>[2x]MSNSYEGCGDLTIFVAVALNKVIGHKNQIPWPHITHDFRFLRNGTTYIPPEVLSKNPDIQNVVIFGRKTYESIPKASLPLKNRINVILSRTVKEVPGCLVYEDLSTAIRDLRANVPHNKIFILGGSFLYKEVLDNGLCDKIYLTRLNKEYPGDTYFPDIPDTFEITAISPTFSTDFVSYDFVIYERKDCKTVFPDPPFDQLLMTGTDISVPKPKYVACPGVRIRNHEEFQYLDILADVLSHGVLKPNRTGTDAYSKFGYQMRFDLSRSFPLLTTKKVALRSIIEELLWFIKGSTNGNDLLAKNVRIWELNGRRDFLDKNGFTDREEHDLGPIYGFQWRHFGAEYLDMHADYTGKGIDQLAEIINRIKTNPNDRRLIVCSWNVSDLKKMALPPCHCFFQFYVSDNKLSCMMHQRSCDLGLGVPFNIASYSILTAMVAQVCGLGLGEFVHNLADAHIYVDHVDAVTTQIARIPHPFPRLRLNPDIRNIEDFTIDDIVVEDYVSHPPIPMAMSA

In this work, we describe the structural features of dihydrofolate reductase-thymidylate synthase from B. bovis (BbDHFR-TS), the causative agent of babesiosis in cattle. BbDHFR-TS is a homodimer that exhibits the classical dimeric interface seen in other structures of ThyA thymidylate synthase and bifunctional DHFR-TS enzymes. This 511-residue, 58.2 kDa bifunctional enzyme consists of a di­hydrofolate reductase (DHFR) subunit at the N-terminus and a thymidylate synthase (TS) subunit at the C-terminus connected by a linker. BbDHFR-TS is an obligate dimer, with two arginine side chains (Arg373′ and Arg374′) from a flexible loop in one protomer making contact with the terminal phosphate of the substrate dUMP in the opposite protomer.

Pemetrexed and raltitrexed are folate analogs designed as antitumour agents and currently approved for use in some countries for treatment of cancer. Depending on the source organism, raltitrexed has a twofold to 50-fold higher activity against TS versus DHFR, while pemetrexed tends to inhibit both enzymes equally well. The two complex structures of BbDHFR-TS have two ligands bound to each subunit of each protomer in the asymmetric unit. When both protomers from each BbDHFR-TS homodimer are compared, the complexed states reveal very similar modes of binding for both drugs to the TS subunit. The pteroyl-like groups of pemetrexed and raltitrexed are parallel to the uracil ring of dUMP when bound, mimicking the pteridine ring of the native cofactor mTHF. Although the ϕ angle of the C-terminal Ala511 in one protomer of the raltitrexed complex is rotated by approximately 30° relative to the other, this has no effect on the virtually identical binding modes of raltitrexed in both TS subunits in a single crystal structure. Both drug molecules are also observed in the DHFR subunit but appear to bind this substrate pocket with different geometries. The bound conformation of pemetrexed is virtually identical in both DHFR protomers but differs slightly from that of raltitrexed, which itself has two different binding modes for its glutamate tail. However, the para-substitution pattern of benzamide in pemetrexed allows the formation of a salt bridge between the α-COOH of its glutamate tail and the Arg83 side chain. Moreover, the glutamate tail of raltitrexed is shifted between protomers of DHFR in the same crystal, with both making hydrogen bonds to Arg42 but only one contacting the N∊ atom of His33. These interactions are not seen for pemetrexed, in which the glutamate group is in essentially the same conformation in both DHFR protomers, despite the differences in side-chain rotamers observed for the nearby Arg39 and Arg42. The antifolate drugs pemetrexed and raltitrexed are capable of binding to the DHFR and TS subunits of BbDHFR-TS, indicating a degree of affinity for both drugs to both folate-binding sites.>[2x]HLIPAQQRTVEHLDAMQWINGDGYLHNVFVRWFNGDVIRPKTWFWQDVKTRKILGWRCDVSENIDSIRLSFMDVVTRYGIPEDFHITIDNTRGAANKWLTGGAPNRYRFKVKEDDPKGLFLLMGAKMHWTSVVAGKGWGQAKPVERAFGVGGL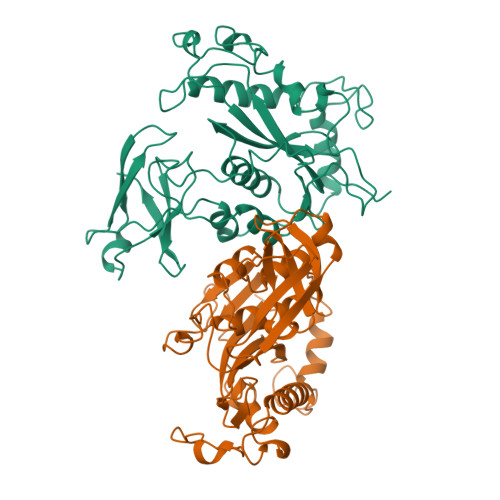EEYVDKHPALAGAYTGPNPQAKPDNYGDRAVDAELFLKTLAEGVAMFNARTGRETEMCGGKLSFDDVFEREYARTIVRKPTEEQKRMLLLPAEAVNVSRKGEFTLKVGGSLKGAKNVYYNMALMNAGVKKVVVRFDPQQLHSTVYCYTLDGRFICEAECLAPVAFNDAAAGREY> IPCGESCVWIPCISSAIGCSCKSKVC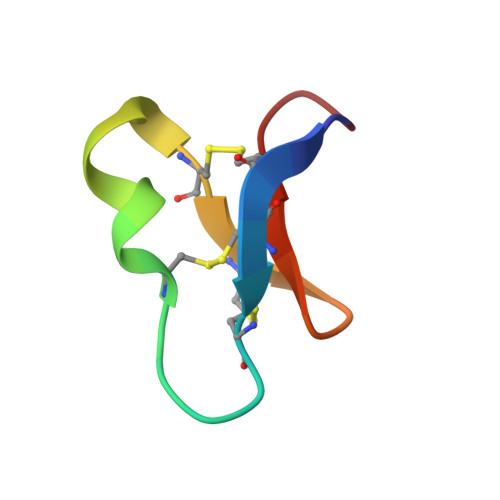YRNG>[2x]DPEFGAGGPWEMRERLGTGGFGNVCLYQHRELDLKIAIKSCRLELSTKNRERWCHEIQIMKKLNHANVVKACDVPEELNILIHDVPLLAMEYCSGGDLRKLLNKPENCCGLKESQILSLLSDIGSGIRYLHENKIIHRDLKPENIVLQDVGGKIIHKIIDLGYAKDVDQGELCTEFVGTLQYLAPELFENKPYTATVDYWSFGTMVFECIAGYRPFLHHLQPFTWHEKIKKKDPKCIFACEEMSGEVRFSSHLPQPNSLCSLIVEPMENWLQLMLNWDPQQRGGPVDLTLKQPRCFVLMDHILNLKIVHILNMTSAKI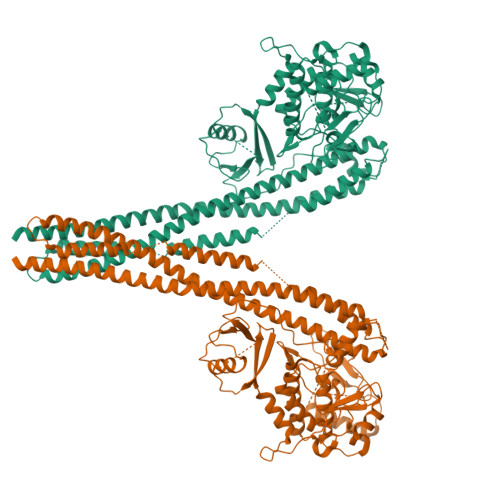ISFLLPPDESLHSLQSRIERETGINTGSQELLSETGISLDPRKPASQCVLDGVRGCDSYMVYLFDKSKTVYEGPFASRSLSDCVNYIVQDSKIQLPIIQLRKVWAEAVHYVSGLKEDYSRLFQGQRAAMLSLLRYNANLTKMKNTLISASQQLKAKLEFFHKSIQLDLERYSEQMTYGISSEKMLKAWKEMEEKAIHYAEVGVIGYLEDQIMSLHAEIMELQKSPYGRRQGDLMESLEQRAIDLYKQLKHRPSDHSYSDSTEMVKIIVHTVQSQDRVLKELFGHLSKLLGCKQKIIDLLPKVEVALSNIKEADNTVMFMQGKRQKEIWHLLKIACTQ>VSEDLRSRIEVLKRKVIEKVQHIQLLQKNVRAQLVDMKRLEVDIDIKIRSCRGSCSRALAREVDLKDYEDQQKQLEQVIAKDLLPSR[4x];>[4x]DNENVVNEYSSELEKHQLYIDETVNSNIPTNLRVLRSILENLRSKIQKLESDVSAQMEYCRTPCTVSCNIPVVSGKECEEIIRKGGETSEMYLIQPDSSVKPYRVYCDMNTENGGWTVIQNRQDGSVDFGRKWDPYKQGFGNVATNTDGKNYCGLPGEYWLGNDKISQLTRMGPTELLIEMEDWKGDKVKAHYGGFTVQNEANKYQISVNKYRGTAGNALMDGASQLMGENRTMTIHNGMFFSTYDRDNDGWLTSDPRKQCSKEDGGGWWYNRCHAANPNGRYYWGGQYTWDMAKHGTDDGVVWMNWKGSWYSMRKMSMKIRPFFPQQ;>MLEEIMKYEASILTHDSSIRYLQEIYNSNNQKIVNLKEKVAQLEAQCQEPCKDTVQIHDITGKDCQDIANKGAKQSGLYFIKPLKANQQFLVYCEIDGSGNGWTVFQKRLDGSVDFKKNWIQYKEGFGHLSPTGTTEFWLGNEKIHLISTQSAIPYALRVELEDWNGR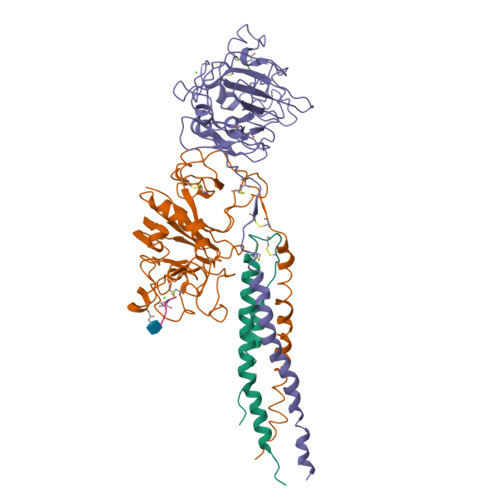TSTADYAMFKVGPEADKYRLTYAYFAGGDAGDAFDGFDFGDDPSDKFFTSHNGMQFSTWDNDNDKFEGNCAEQDGSGWWMNKCHAGHLNGVYYQGGTYSKASTPNGYDNGIIWATWKTRWYSMKKTTMKIIPFNRLTIGEGQQHHLGGAKQAGDV[4x];>GPRPX[8x]>[2x]MERTDIRMAIVADHLGLSWTELARELNFSVDEIN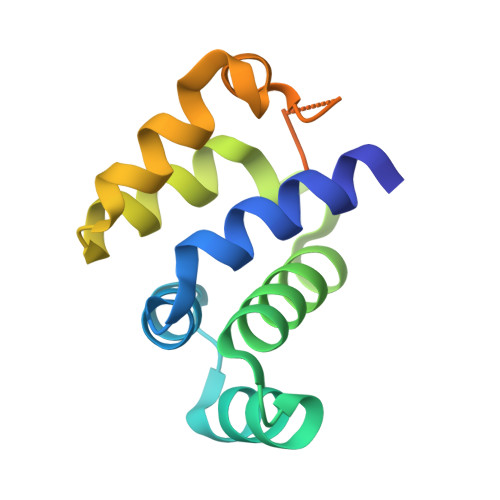QIRVENPNSLISQSFMLLKKWVTRDGKNATTDALTSVLTKINRIDIVTLLEGPIFDYGNISGTRSFADENNVFHDPVDGLEHHHHHH> HK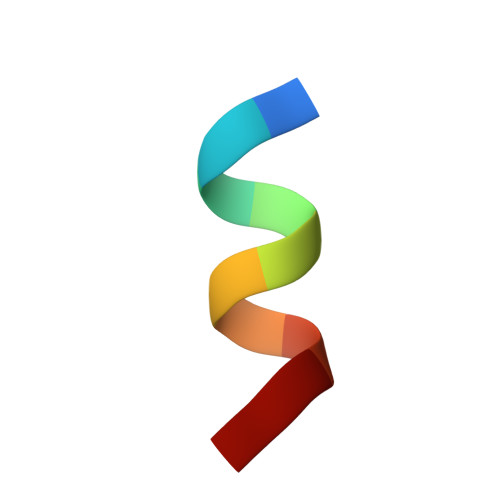ILHRLLQD> NNAFCAGFGLSCKWECWCTAHGTGNELRYATAAGCGDHLSKSYYDARAGHCLFSDDLRNQFYSHCSSLNNNMSCRSLSKR;> GKRPRPVMCQCVDTTNGGVRLDAVTRAACSIDSFIDGYY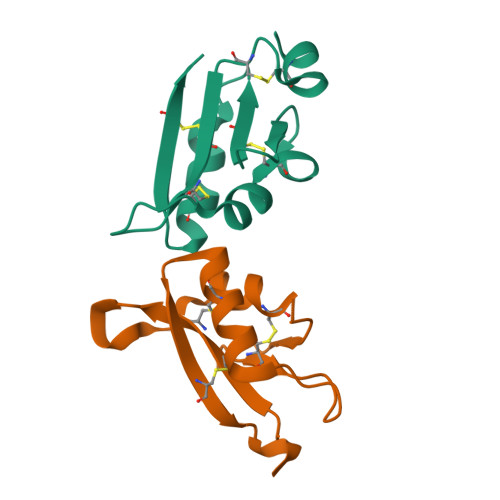TEKDGFCRAKYSWDLFTSGQFYQACLRYSHAGTNCQPDPQYE> MRGSAHVVILGAGTGGMPAAYEMKEALGSGHEVTLISANDYFQFVPSNPWVGVGWKERDDIAFPIRHYVERKGIHFIAQSAEQIDAEAQNITLADGNTVHYDYLMIATGPKLAFENVPGSDPHEGPVQSICTVDHAERAFAEYQALLREPGPIVIGAMAGASCFGPAYEYAMIVASDLKKRGMRDKIPSFTFITSEPYIGALGIQGVGDSKGILTKGLKEEGIEAY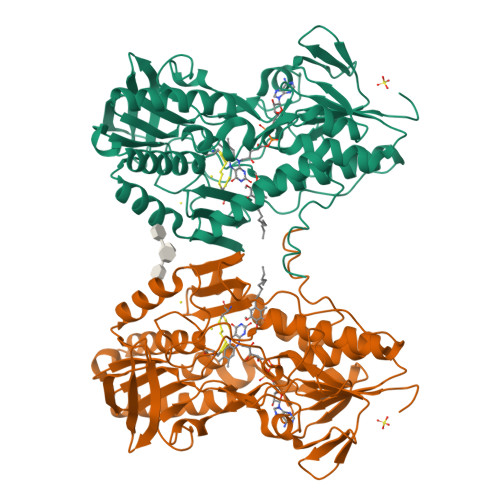TNCKVTKVEDNKMYVTQVDEKGETIKEMVLPVKFGMMIPAFKGVPAVAGVEGLCNPGGFVLVDEHQRSKKYANIFAAGIAIAIPPVETTPVPTGAPKTGYMIESMVSAAVHNIKADLEGRKGEQTMGTWNAVCFADMGDRGAAFIALPQLKPRKVDVFAYGRWVHLAKVAFEKYFIRKMKMGVSEPFYEKVLFKMMGITRLKEEDTHRKAS>[2x]ADPSEHCSHMIGNGHLKVLQQLIDSQMETSCQIAFEFVDQEQLDDPVCYLKKAFFLVQDIIDETMRFKDNTPNANATERLQELSNNLNSCFTKDYEEQNK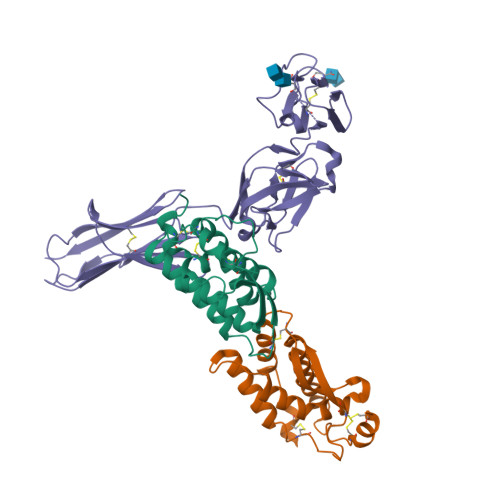ACVRTFHETPLQLLEKIKNFFNETKNLLEKDWNIFTKNCNNSFAKCSSHHHHHHH;> ADPAPVIEPSGPELVVEPGETVTLRCVSNGSVEWDGPISPYWTLDPESPGSTLTTRNATFKNTGTYRCTELEDPMAGSTTIHLYVKDPAHSWNLLAQEVTVVEGQEAVLPCLITDPALKDSVSLMREGGRQVLRKTVYFFSPWRGFIIRKAKVLDSNTYVCKTMVNGRESTSTGIWLKVNRVHPEPPQIKLEPSKLVRIRGEAAQIVCSATNAEVGFNVILKRGDTKLEIPLNSDFQDNYYKKVRALSLNAVDFQDAGIYSCVASNDVGTRTATMNFQVVESHHHHHHH The ubiquitin specific protease 7 (USP7), also known as herpes virus associated ubiquitin specific protease (HAUSP), is a well-characterized deubiquitinase. USP7 plays important roles in various biological processes, including cell survival, proliferation, apoptosis, tumorigenesis, viral infection, and epigenetic regulation through regulating the protein stability of tumor suppressors (p53, PTEN, FOXO, claspin), E3 ligases (MDM2, Mule, viral proteins ICP0), epigenetic regulators (DNMT1, Tip60, UHRF1). USP7 is comprised of three recognizable domains: the N-terminal TRAF domain, the catalytic domain, and the C-terminal Tandem UBL domain (designated TUDUSP7). To test this hypothesis, we first investigated the interaction between USP7 and the Herpes simplex virus type 1 (HSV1) regulatory protein ICP0 (also known as Vmw110), which is the first identified USP7-interacting protein and regulates the lytic and latent viral infection through inducing proteasomal degradation of various cellular proteins.

To investigate how ICP0 binds to TUDUSP7, we determined the crystal structure of TUDUSP7 in complex with ICP0 (613–633) at 2.70 Å resolution. As observed in previous studies, UBL1–2, UBL3, and UBL4–5 of TUDUSP7 form three separate modules and are connected by flexible regions flanking the UBL3. The ICP0 packs against an acidic groove on the surface of UBL1–2. As indicated in the TUDUSP7-ICP0 structure, the interaction is mediated by a network of hydrogen bonds and salt bridge contacts. Residue K620ICP0 forms hydrogen bonds with the carbonyl oxygen atoms of residues K681USP7, D684USP7 and side chain of D762USP7. Residue K624ICP0 snugly inserts into an acidic cavity, with the side chain stabilized by residues E759USP7 and D764USP7. Residues R626ICP0 and H627ICP0 form hydrogen bonds with side chain of residue D758USP7. Consistent with the observation from the structural analyses, mutations K624AICP0 (1KA) and K620A/K624AICP0 (2KA) of ICP0, largely decreased the binding affinities to TUDUSP7, compared with the wild-type ICP0, supporting the key role of these residues in mediating the intermolecular interaction. Structural comparison of USP7-DNMT1 and USP7-ICP0 indicates that ICP0 and KG-LinkerDNMT1 pack against the same acidic pocket of TUDUSP7 in an opposite orientation. Taken together, USP7 binds to distinct proteins on two separate sites, TRAF and the acidic pocket on TUDUSP7, respectively.

> GPLGSEAHLYMQVQIVAEDQFCGHQGNDMYDEEKVKYTVFKVLKNSSLAEFVQSLSQTMGFPQDQIRLWPMQARSNGTKRPAMLDNEADGNKTMIELSDNENPWTIFLETVDPELAASGATLPKFDKDHDVMLFLKMYDPKTRSLNYCGHIYTPISCKIRDLLPVMCDRAGFIQDTSLILYEEVKPNLTERIQDYDVSLDKALDELMDGDIIVFQKDDPENDNSELPTAKEYFRDLYHRVDVIFCDKTIPNDPGFVVTLSNRMNYFQVAKTVAQRLNTDPMLLQFFKSQGYRDGPGNPLRHNYEGTLRDLLQFFKPRQPKKLYYQQLKMKITDFENRRSFKCIWLNSQFREEEITLYPDKHGCVRDLLEECKKAVELGEKASGKLRLLEIVSYKIIGVHQEDELLECLSPATSRTFRIEEIPLDQVDIDKENEMLVTVAHFHKEVFGTFGIPFLLRIHQGEHFREVMKRIQSLLDIQEKEFEKFKFAIVMMGRHQYINEDEYEVNLKDFEPQPGNMSHPRPWLGLDHFNKAPKRSRYTYLEKAIKIHN;> SGPRGPRKCARKTRHAETSGA>[2x]PVNPCCYYPCQHQGICVRFGLDRYQCDCTRTGYSGPNCTIPEIWTWLRTTLRPSPSFIHFLLTHGRWLWDFVNATFIRDTLMRLVLTVRSNLIPSPPTYNIAHDYISWESFSNVSYYTRILPSVPRDCPTPMDTKGKKQLPDAEFLSRRFLLRRKFIPDPQSTNLMFAFFAQHFTHQFFKTSGKMGPGFTKALGHGVDLGHIYGDNLERQYQLRLFKDGKLKYQMLNGEVYPPSVEEAPVLMHYPRGIPPQSQMAVGQEVFGLLPGLMLYATIWLREHNRVCDLLKAEHPTWGDEQLFQTARLILIGETIKIVIEEYVQQLSGYFLQLKFDPELLFGAQFQYRNRIAMEFNQLYHWHPLMPDSFRVGPQDYSYEQFLFNTSMLVDYGVEALVDAFSRQPAGRIGGGRNIDHHILHVAVDVIKESRVLRLQPFNEYRKRFGMKPYTSFQELTGEKEMAAELEELYGDIDALEFYPGLLLEKCHPNSIFGESMIEMGAPFSLKGLLGNPICSPEYWKASTFGGEVGFNLVKTATLKKLVCLNTKTCPYVSFHVPD

COX inhibitors are among the most prominent categories of compounds in the drug market and are categorized into the class of traditional NSAIDs that inhibit both COX‐1 and COX‐2, as well as into the class of COX‐2‐specific inhibitors, referred to as coxibs. COX‐1 dominates prostanoid formation in monocytes and platelets, with the latter exclusively expressing COX‐1 but not COX‐2. COX‐1 crystallizes as a homodimer in the asymmetric unit, consisting of two ≈72 kDa subunits tightly packed against each other via an extensive binding interface of ≈2500 Å2. Previous studies have revealed that small‐molecule NSAIDs interact with the proximal and central inhibitor binding side of COX, which both overlap with the binding pocket for arachidonic acid.

To determine the binding mode and rationalize these biochemical effects, we determined the crystal structure of the ovine COX‐1 (oCOX‐1) in complex with the subtype‐selective derivative 2a (oCOX‐1 IC50 = 0.160 ± 0.001 µm, inactive on hCOX‐2). Compound 2a was identified in an unbiased Fo–Fc polder map within the oCOX‐1 hydrophobic channel between residues Arg120 and Tyr355. The methoxyacetate residue of compound 2a was the only part of the molecule that did not have a clear density in the crystal structure, possibly underscoring its flexibility and lack of binding interactions. The crystal structure revealed that the inhibitor resided in the active site of the enzyme in an almost planar conformation. Compound 2a bound to the substrate channel with one chlorobenzene facing Ser530, and another chlorobenzene facing down near residues Tyr355 and Arg120, the entry point to the active site. The ligand was engaged in two sets of interactions with oCOX‐1 residues, namely a hydrogen bridge between a chlorine atom of the ligand and the hydroxyl group of residue Ser530, and multiple non‐bonded van der Waals and hydrophobic contacts with 19 oCOX‐1 residues. The ligand portion in the distal binding pocket was surrounded by hydrophobic residues (Leu531, Leu534, Leu535, Ile345, Met113) and formed van der Waals interactions with Lys360. All three compounds interacted with the catalytic Ser530 and structurally overlapped in this central part, whereas compound 2a adopted an inverted orientation, occupying a hydrophobic protein pocket lined by residues Met113, Val116, Ile345, Lys360, Leu531, Leu534, and Leu535. This binding pose mimics the bound state of the endogenous substrate arachidonic acid. Compound 2a inhibited COX‐1 independently of the arachidonic acid concentration in a highly potent manner, which was confirmed in wash‐out experiments indicating tight binding.Within Sulfolobales, member species encode for three types of T4P, namely the archaellum, the UV-inducible pilus system (Ups) and the archaeal adhesive pilus (Aap). Whereas the archaellum functions primarily in swimming motility, and the Ups in UV-induced cell aggregation and DNA-exchange, the Aap plays an important role in adhesion and twitching motility. Here, we determine the structure of the Aap, and show that it is solely composed of multiple copies of AapB. Each AapB subunit consists of an N-terminal α-helix tail, followed by a globular (head) domain.

Here we present the structure of the Aap pilus from S. acidocaldarius at 3.2 Å resolution. Aided by the building of an initial atomic model, this map was sufficient to deduce the helical parameters, which we identified as a helical twist of −39.9° and a rise of 15.4 Å. Careful analysis of the filament’s structure revealed that the AapB monomers exist in three distinct conformations (henceforth designated as conformations A, B and C) These differ in the angle between the head and the tail domain with values of ~112°, 129°, and 121° for conformations A, B and C, respectively. Each distinct conformation repeats along one of the three left-handed 3-start helices of the pilus, meaning that each of these 3-start helices harbours exclusively one of the three conformations. In conformation A and B this hinge is short and lies between G51, the final amino acid of the α helix and I53, the first amino acid of β1. In conformation C, the hinge region spans from I53 to I47, across a stretch of four additional amino acids where the α-helix is “melted” into a loop. Moreover, the distinct hinge of conformation C causes the tail domain to stretch out, meaning that it reaches further into the centre of the filament. Interestingly, the α-helical tails within the core of the S. acidocaldarius Aap are significantly curved, with the concave side of each α-helix facing the filament’s periphery. The glycan densities originated from asparagine residues, (N48, N60, and N88), which were all part of a consensus N-glycosylation sequon (NXS/T). While all six sugar units of the hexasaccharide were resolved in the threads, the map of the Aap contained only densities for the first one or two sugar residues.

>[72x]LSGAIVALILVIAGVIIAIAVVLFAFGLIPGISNQGSIQVLGSGTITNSTASGSSRTIYNITITVKNTGTTSISVTSININGQPFNINGTAPSIPAGRTQPITFEVTPASGKPNFSPGASYTATIYFSNGQGAPATLIYQG(2~{S})-2-[[(2~{S})-4-methyl-1-oxidanyl-1-oxidanylidene-pentan-2-yl]oxycarbonylamino]pentanedioic 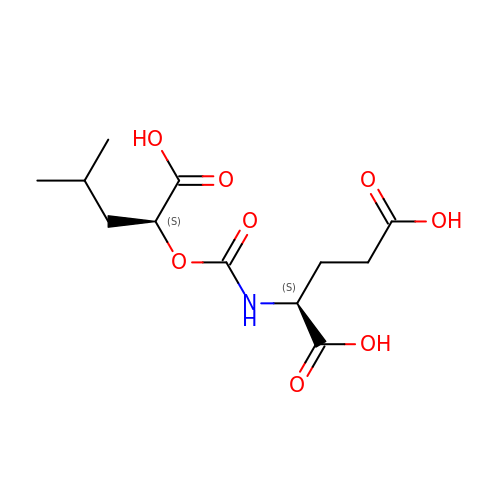acid | C12 H19 N O8 | GCAXQXOSZUNUBK-YUMQZZPRSA-N> 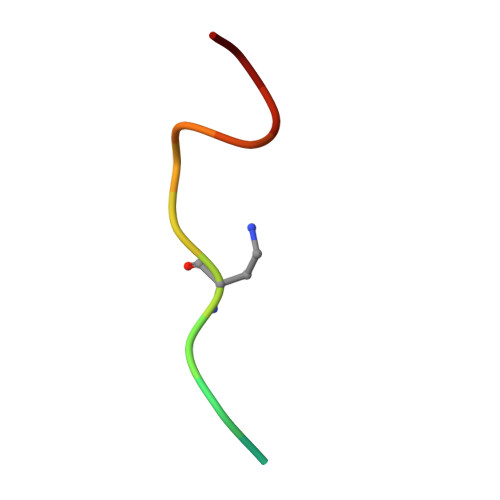GRKRRQASMTEFYH> MAL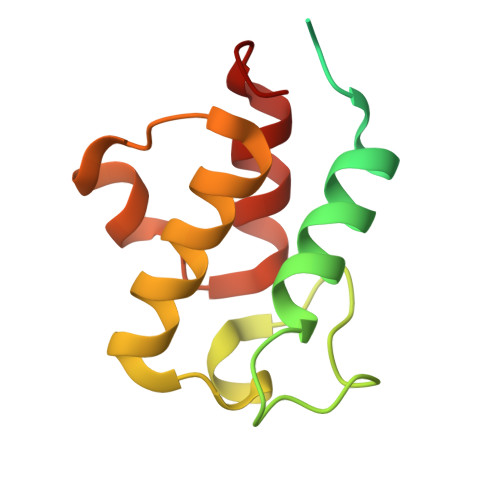SSASSFFKAVVLRNLRVSVSQSTFVPIGNVISRAYGGHGLDRDTVTERVIHVAKHFEKVDPNKITPTATFEELGLDSLDTVELVMALEEEFGLEIPDNEADKITTMADAISYVVSNPLAK> SDEFDALRIKWATLLTGGPALDPADSDIAARTDKLAQDANDYWEDMDLSSSRTYIWYALRGNGTSDNVNAVYERLRTMALAATTVGSSLYGNADLKEDILDALDWLYVNSYNSTRSRSAYNWWHWQLGIPMSLNDIAVLLYDDISAARMATYMDTIDY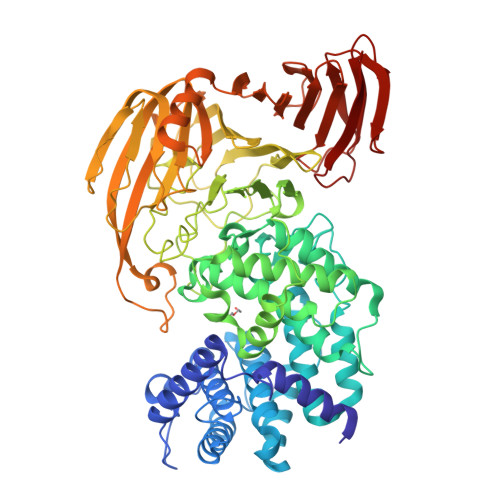FTPSIGLTGANRAWQAIVVGVRAVIVKDAVKLAAARNGLSGTGIFPYATGGDGFYADGSFVQHTTFAYTGGYGSSVLETTANLMYLLSGSTWSVSDPNQSNVWQWIYEAYRPLLYKGAMMDMVRGREISRSYAQDHAVGHGIVASIVRLAQFAPAPHAAAFKQIAKRVIQEDTFSSFYGDVSTDTIRLAKAIVDDPSIAPAAAPNLYKQYAAMDRAVLQRPGFALGLALYSTRISSYESINSENGRGWYTGAGATYLYNQDLAQYSEDYWPTVDAYRIPGTTVASGTPIASGTGTSSWTGGVSLAGQYGASGMDLSYGAYNLSARKSWFMFDDEIVALGSGISSTAGIPIETVVDNRKLNGAGDNAWTANGAALSTGLGVAQTLTGVNWVHLAGNTADGSDIGYYFPGGATLQTKREARTGTWKQINNAPATPSTAVTRNYETMWIDHGTNPSGASYGYVLLPNKTSAQVGAYAADPAIEIVVNTSGVQSVKEKTLGLVGANFWTDTTQTADLITSNKKASVMTREIADERLEASVSDPTQANNGTIAIELARSAEGYSADPGITVTQLAPTIKFTVNVNGAKGKSFHASFQLG> MKKLIPILEKIPEVELPVKEITFKEKLKWTGIVLVLYFIMGCIDVYTAGAQIPAIFEFWQTITASRIGTLITLGIGPIVTAGIIMQLLVGSGIIQMDLSIPENRALFQGCQKLLSIIMCFVEAVLFVGAGAFGILTPLLAFLVIIQIAFGSIILIYLDEIVSKYGIGSGIG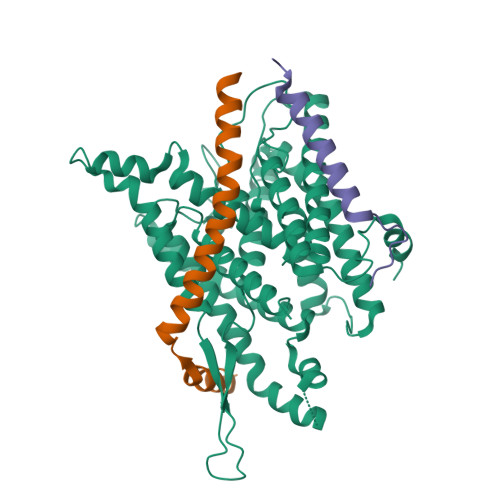LFIAAGVSQTIFVGALGPEGYLWKFLNSLIQGVPNIEYIAPIIGTIIVFLMVVYAECMRVEIPLAHGRIKGAVGKYPIKFVYVSNIPVILAAALFANIQLWGLALYRMGIPILGHYEGGRAVDGIAYYLSTPYGLSSVISDPIHAIVYMIAMIITCVMFGIFWVETTGLDPKSMAKRIGSLGMAIKGFRKSEKAIEHRLKRYIPPLTVMSSAFVGFLATIANFIGALGGGTGVLLTVSIVYRMYEQLLRERTSELHPAIAKLLNK;> MKTDFNQKIEQLKEFIEECRRVWLVLKKPTKDEYLAVAKVTALGISLLGIIGYIIHVPATYIKGILKPPTTPRV;> MSKREETGLATSAGLIRYMDETFSKIRVKPEHVIGVTVAFVIIEAILTYGRFL> MAKFFIDRPIFAWVISIFIIAAGIFGIKSLPVSQYPSVAAPTITLHAIYPGASAQVMEGSVLSVIERNMNGVEGLDYMSTSADSSGSGSVSLTFTPDTDENLAQVEVQNKLSEVLSTLPATVQQYGVTVSKARSNFLMIVMLSSDVQSTEEMNDYAQRNVVPELQRIEGVGQVRLFGAQRAMRIWVDPKKLQNYNLSFADVGSALSAQNIQISAGSIGSLPAVRGQTVTATVTAQGQLGTAEEFGNVILRANTDGSNIYLKDVAKVGLGMEDYSSSTRLNGVNTTGMAVMLSNSGNAMATAKAVKERLAVLEKYFPQGMSWKTPYDTSKFVEISIEKVIHTLIEAMV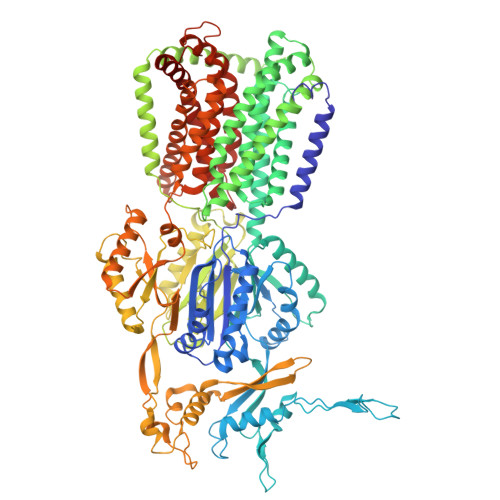LVFVVMYLFLQNIRYTLIPTIVVPISLLGGFAFISYMGMSINVLTMFAMILVIGIVVDDAIVVVENVERIMAGEGLPPKEATKKAMGQISGAVIGITAVLISVFVPLAMFSGAAGNIYKQFALTMASSIAFSAFLALTLTPALCATMLKTIPKGHHEEKKGFFGWFNKKFDSWTHGYEGRVAKVLRKTFRMMVVYIGLAVVGVFLFMRLPTSFLPTEDQGFVMVSVQLPAGATKERTDATLAQVTQLAKSIPEIENIITVSGFSFSGSGQNMAMGFAILKDWNERTASGSDAVAVAGKLTGMMMGTLKDGFGIAVVPPPILELGNGSGLSINLQDRNNTGHTALLAKRNELIQKMRASGLFDPSTVRAGGLEDSPQLKIDINRAAAAAQGVSFADIRTALASALSSSYVSDFPNQGRLQRVMVQADGDARMQPADILNLTVPNSSGIAVPLSSIATVSWQMGTEQSVRFNGYPAMELSGSPATGVSTGQAMEAVQKMVDELGSGYSLEWGGQSREEAKGGSQTIALYALAAVAVFLVLAALYESWSIPLAVLLVMPLGLAGAAAGVTGRNLFEGLLGSVPSFANDIYFQVGFVTVMGLSAKNAILIIEFAKDLQAQGKSAVEAALEAARLRFRPIIMTSFAFILGVVPLYIAGGASSASQRAIGTTVFWGMLIGTLLSVFLVPLFYVVVRKFFKETAHE>[8x]MTMTLAKRFTAEVVGTFILVFFGPGAAVITLMIANGADKPN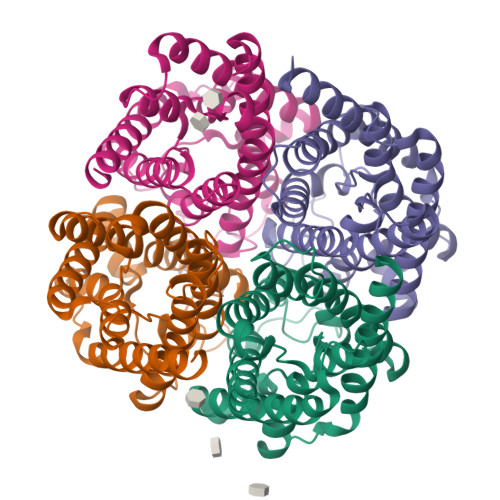EFNIGIGALGGLGDWFAIGMAFALAIAAVIYSLGRISGAHINPAVTIALWSIGRFPGREVVPYIVAQFIGAALGSLLFLACVGPAAATVGGLGATAPFPGIGYGQAILTEAIGTFLLMLVIMGVAVDERAPPGFAGLVIGLTVGGIITTIGNITGSSLNPARTFGPYLGDSLMGINLWQYFPIYVIGPIVGAVAAAWLYNYLAKE> SGPGFDFAQAIMKKNTVIARTEKGEFTMLGVYDRVAVIPTHASVGETIYINDVETKVLDACALRDLTDTNLEITIVRLDRNQKFRDIRHFLPRYEDDYNDAVLSVHTSKFPNMYIPVGQVTNYGFLNLG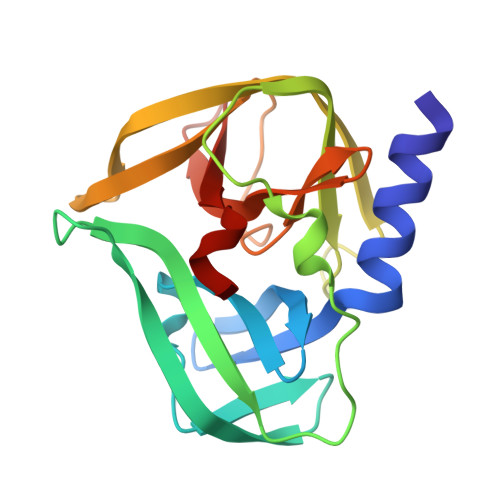GTPTHRILMYNFPTRAGQAGGVVTTTGKVIGIHVGGNGAQGFAAMLLHSYFSD>GQSNSNNWRWFDDRSGRWCSYSASNNSTIDSAWKSGETSVRFTAGRRRYTVQFTTMVQVNEETGNRRPVMLTLLRVPRLNKNSKNSNGQEL[4x]

The WWE domain is a relatively under-researched domain found in twelve human proteins and characterized by a conserved tryptophan-tryptophan-glutamate (WWE) sequence motif. Six of these WWE domain-containing proteins also contain domains with E3 ubiquitin ligase activity. Here, we present novel crystal structures of the HUWE1, TRIP12, and DTX1 WWE domains in complex with PAR building blocks and their analogs, thus enabling a comprehensive analysis of the PAR binding site structural diversity. A highly conserved feature in all determined structures is the recognition and therefore the interactions involving the adenine ring of the ligands.

Unlike RNF146 WWE, the single domain WWE family members HUWE1 and TRIP12 exhibit higher potency for ADPr over iso-ADPr in our binding assays. The HUWE1-ADPr and TRIP12-ADP crystal structures revealed high conservation of the ligand-binding sites, with most of the ligand interactions being conserved. The phosphate groups of the two ligands occupy pockets with favorable polar and positively charged groups, interacting with Tyr1658, Asn1669, Thr1672, Asn1674, and Arg1676 in HUWE1 and Tyr809, Asn820, Thr823, Thr825, Arg827 in TRIP12. Despite the terminal ribose having electron density in the HUWE1-ADPr structure, it points towards the protein surface with no additional directed protein–ligand interactions, indicating that the ADP moiety may be the smallest unit that HUWE1 and TRIP12 recognize. Firstly, Tyr107 that makes a key interaction with the distal ribose oxygen of iso-ADPr in RNF146, is replaced by tryptophans in HUWE1 (Trp1619) and TRIP12 (Trp771)—the tryptophans would be incapable of making a similar interaction with iso-ADPr. Secondly, the region interacting with the distal phosphate of iso-ADPr in RNF146 contains suitable polar and positively charged residues, while the corresponding region in HUWE1 and TRIP12 contain some acidic residues including two aspartic acids (1621–1622 in HUWE1 and 773–774 in TRIP12), making it less positively charged, and therefore less favorable for potential interactions with the distal phosphate moiety of iso-ADPr, explaining the lower iso-ADPr potencies observed. Taken together, structural and affinity data suggest that the WWE pocket of HUWE1 and TRIP12 recognize the terminal ADP moiety of PAR, rather than the iso-ADPr moiety as described for RNF146. An overlay of the TRIP12-ADP and HUWE1-ADPr structures show a highly conserved ADP binding site, with the substitution of Thr825 in TRIP12 with Asn1674 in HUWE1 being one of the small differences. A mutation of Asn1674 to threonine in HUWE1 had no effect on PAR11-mer binding, indicating that the potency of PAR binding is determined by factors outside of the ligand-binding pocket, possibly including the PAR polymer structure.> MLGTGPAAATTAATTSXXXXXXXXXXXXXXSRNEETXXXXXXXXXXXXXXXXXEMSQEEXTRFYDQLNHHIFELVSSSDANERKGGILAIASLIGVEGGNATRIGRFANYLRNLLPSNDPVVMEMASKAIGRLAMAGDTFTAEYVEFEVKRALEWLGADRNEGRRHAAVLVLRELAISVPTFFFQQVQPFFDNIFVAVWDPKQAIREGAVAALRACLILTTQREPKEMQKPQWYRHTFEEAEKGFDETLAKEKGMNRDDRIHGALLILNELVRISSMEGERLREEMEEITQQQLVHDKYCKDLMGFGTKPRHITPFTSFQAVQPQQSNALVGLLGYSSHQGLMGFGTSPSPAKSTXXXXXXXXXXXXXXXXXXXXXXXXXRNSKNSLIQMTILNLLPRLAAFRPSAFTDTQYLQDTMNHVLSCVKKEKERTAAFQALGLLSVAVRSEFKVYLPRVLDIIRAALPPKDFAHKRQKAMQVDATVFTCISMLARAMGPGIQQDIKELLEPMLAVGLSPALTAVLYDLSRQIPQLKKDIQDGLLKMLSLVLMXKPLRHPGMPKGLAHQLASPGLTTLPEASXVGSITLALRTLGSFEFEGHSLTQFVRHCADHFLNSEHKEIRMEAARTCSRLLTPSIHLISGHAHVVSQTAVQVVADVLSKLLVVGITDPDPDIRYCVLASLDERFDAHLAQAENLQALFVALNDQVFEIRELAICTVGRLSSMNPAFVMPFLRKMLIQILTELEHSGIGRIKEQSARMLGHLVSNAPRLIRPYMEPILKALILKLKDPDPDPNPGVINNVLATIGELAQVSGLEMRKWVDELFIIIMDMLQDSSLLAKRQVALWTLGQLVASTGYVVEPYRKYPTLLEVLLNFLKTEQNQGTRREAIRVLGLLGALDPYKHKVNIGMIDQSRDASAVSLSESKSSQDSSDYSTSEMLVNMGNLPLDEFYPAVSMVALMRIFRDQSLSHHHTMVVQAITFIFKSLGLKCVQFLPQVMPTFLNVIRVCDGAIREFLFQQLGMLVSFVKSHIRPYMDEIVTLMREFWVMNTSIQSTIILLIEQIVVALGGEFKLYLPQLIPHMLRVFMHDNSPGRIVSIKLLAAIQLFGANLDDYLHLLLPPIVKLFDAPEAPLPSRKAALETVDRLTESLDFTDYASRIIHPIVRTLDQSPELRSTAMDTLSSLVFQLGKKYQIFIPMVNKVLVRHRINHQRYDVLICRIVKGYTLADEEEDPLIYQHRMLRSGQGDALASGPVETGPMKKLHVSTINLQKAWGAARRVSKDDWLEWLRRLSLELLKDSSSPSLRSCWALAQAYNPMARDLFNAAFVSCWSELNEDQQDELIRSIELALTSQDIAEVTQTLLNLAEFMEHSDKGPLPLRDDNGIVLLGERAAKCRAYAKALHYKELEFQKGPTPAILESLISINNKLQQPEAAAGVLEYAMKHFGELEIQATWYEKLHEWEDALVAYDKKMDTNKDDPELMLGRMRCLEALGEWGQLHQQCCEKWTLVNDETQAKMARMAAAAAWGLGQWDSMEEYTCMIPRDTHDGAFYRAVLALHQDLFSLAQQCIDKARDLLDAELTAMAGESYSRAYGAMVSCHMLSELEEVIQYKLVPERREIIRQIWWERLQGCQRIVEDWQKILMVRSLVVSPHEDMRTWLKYASLCGKSGRLALAHKTLVLLLGVDPSRQLDHPLPTVHPQVTYAYMKNMWKSARKIDAFQHMQHFVQTMQQQAQHAIATEDQQHKQELHKLMARCFLKLGEWQLNLQGINESTIPKVLQYYSAATEHDRSWYKAWHAWAVMNFEAVLHYKHQNQARDEKKKLRHASGANITNATTAATTAATATTTASTEGSNSESEAESTENSPTPSPLQKKVTEDLSKTLLMYTVPAVQGFFRSISLSRGNNLQDTLRVLTLWFDYGHWPDVNEALVEGVKAIQIDTWLQVIPQLIARIDTPRPLVGRLIHQLLTDIGRYHPQALIYPLTVASKSTTTARHNAANKILKNMCEHSNTLVQQAMMVSEELIRVAILWHEMWHEGLEEASRLYFGERNVKGMFEVLEPLHAMMERGPQTLKETSFNQAYGRDLMEAQEWCRKYMKSGNVKDLTQAWDLYYHVFRRISKQLPQLTSLELQYVSPKLLMCRDLELAVPGTYDPNQPIIRIQSIAPSLQVITSKQRPRKLTLMGSNGHEFVFLLKGHEDLRQDERVMQLFGLVNTLLANDPTSLRKNLSIQRYAVIPLSTNSGLIGWVPHCDTLHALIRDYREKKKILLNIEHRIMLRMAPDYDHLTLMQKVEVFEHAVNNTAGDDLAKLLWLKSPSSEVWFDRRTNYTRSLAVMSMVGYILGLGDRHPSNLMLDRLSGKILHIDFGDCFEVAMTREKFPEKIPFRLTRMLTNAMEVTGLDGNYRITCHTVMEVLREHKDSVMAVLEAFVYDPLLNWRLMDTNTKGNKRSRTRTDSYSAGQSVEILDGVELGEPAHKKTGTTVPESIHSFIGDGLVKPEALNKKAIQIINRVRDKLTGRDFSHD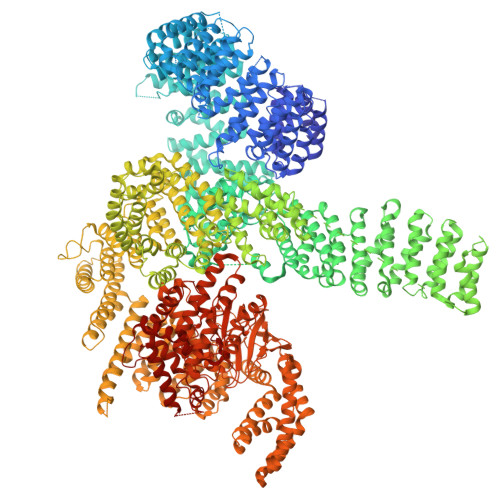DTLDVPTQVELLIKQATSHENLCQCYIGWCPFW>[18x]SAREEQVTSEQAKFWL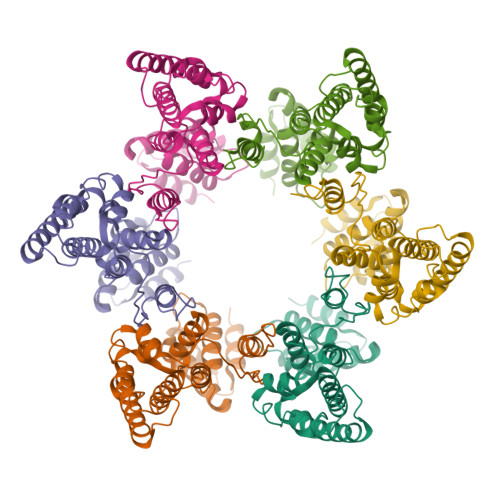GLGGGRVSPPGPECIEKPATERRIDKGEEVGETTVQRDAKMAPEETATPKTVGTSCYHCGTAIGCNCATASAPPPPYVGSGLYPSLAGVGEQQGQGGDTPPGAEQSRAEPGHAGQAPGPALTDWARVREELASTGPPVVAMPVVIKTEGPAWTPLEPKLITRLADTVRTKGLRSPITMAEVEALMSSPLLPHDVTNLMRVILGPAPYALWMDAWGVQLQTVIAAATRDPRHPANGQGRGERTNLNRLKGLADGMVGNPQGQAALLRPGELVAITASALQAFREVARLAEPAGPWADIMQGPSESFVDFANRLIKAVEGSDLPPSARAPVIIDCFRQKSQPDIQQLIRTAPSTLTTPGEIIKYVLDRQKTAPLTDQGIAAAMSSAIQPLIMAVVNRERDGQTGSGGRARGLCYTCGSPGHYQAQCPKKRKSGNSRERCQLCNGMGHNAKQCRKRDGNQGQRPGKGLSSGPWPGPEQPAVS>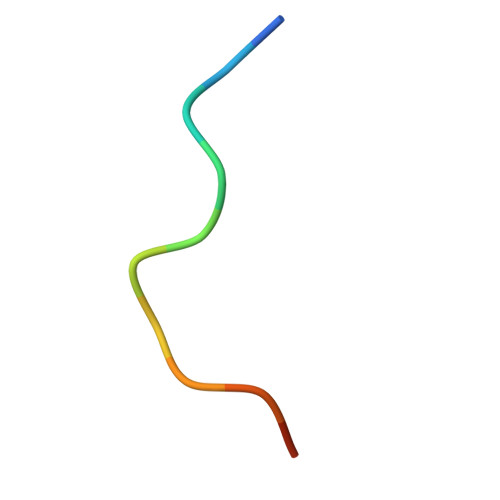 PPPRPTAPKPLL> GSHMDSTTIQQNKDTLSQIVVFPTGNYDKNEANAMVNRLANIDGKYLNALKQNNLKIK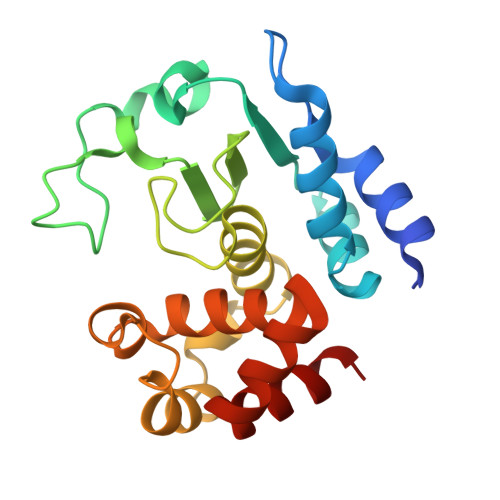LLSGKLTDEKEYAYLKGVVPKGWEGTGKTWDDVPGLGGSTVALRIGFSNKGKGHDAINLELHATAHAIDHIVLNDISKSAQFKQIFAKEGRSLGNVNFLGVYPAEFFAESFAYYYLNQDTNSKLKSACPQTYSFLQNLAK>MVLKRKGLLIILDGLGDRPIKELNGLTPLEYANTPNMDKLAEIGILGQQDPIKPGQPAGSDTAHLSIFGYDPYETYRGRGFFEALGVGLDLSKDDLAFRVNFATLENGIITDRRAGRISTEEAHELARAIQEEVDIGVDFIFKGATGHRAVLVLKGMSRGYKVGDNDPHEAGKPPLKFSYEDEDSKKVAEILEEFVKKAQEVLEKHPINERRRKEGKPIANYLLIRGAGTYPNIPMKFTEQWKVKAAGVIAVALVKGVARAVGFDVYTPEGATGEYNTNEMAKAKKAVELLKDYDFVFLHFKPTDAAGHDNKPKLKA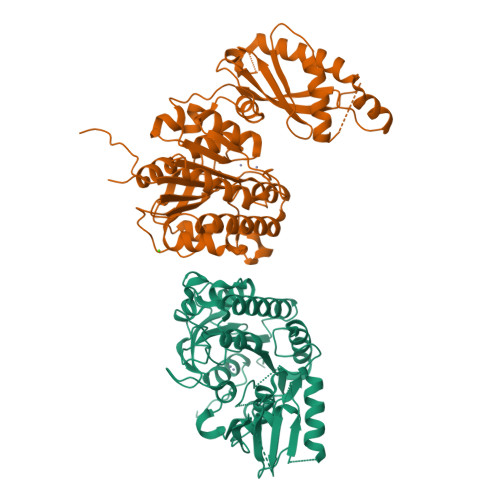ELIERADRMIGYILDHVDLEEVVIAITGDHSTPCEVMNHSGDPVPLLIAGGGVRTDDTKRFGEREAMKGGLGRIRGHDIVPIMMDLMNRSEKFGA[2x]> MLRDLFDRAVVLSHYIANLSSEMFSE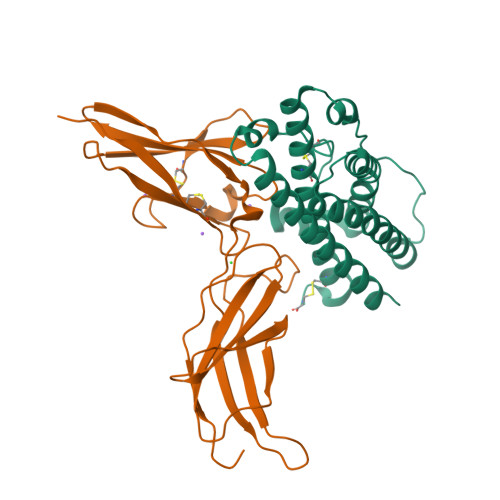FDKRYTHGRGFITKAINSCHTSSLATPEDKEQAQQMNQKDFLSLIVSILRSWNEPLYHLVTEVRGMQEAPEAILSKAVEIEEQTKRLLERMELIVSQVHPETKENEIYPVWSGLPSLQMADEESRLSAYYNLLHCLRRDSHKIDNYLKLLKCRIIHNNNC;> MLPPGKPEIFKCRSPNKETFTCWWRPGTDGGLPTNYSLTYHREGETLMHECPDYITGGPNSCHFGKQYTSMWRTYIMMVNATNQMGSSFSDELYVDVTYIVQPDPPLELAVEVKQPEDRKPYLWIKWSPPTLIDLKTGWFTLLYEIRLKPEKAAEWEIHFAGQQTEFKILSLHPGQKYLVQVRCKPDAGYWSAWSPATFIQIPSDFTMND>[2x]FPDGTLGMDAAVQEDHDNGTQLDSLTLASINTDFAFSLYKELVLKNPDTNIVFSPLSISAALALVSLGAKGNTLEEILEGLKFNLTETSEADIHQGFGHLLQRLNQPKDQVQISTGS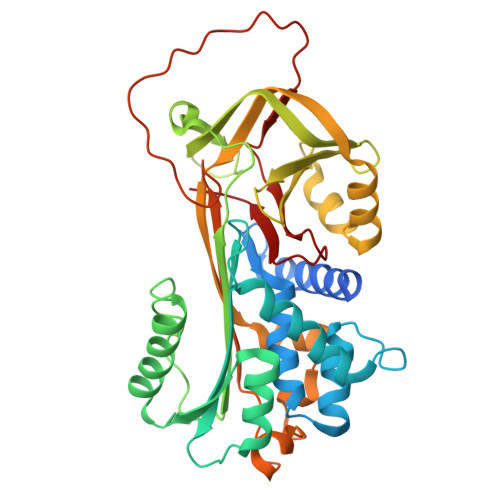ALFIEKRQQILTEFQEKAKTLYQAEAFTADFQQPRQAKKLINDYVRKQTQGMIKELVSDLDKRTLMVLVNYIYFKAKWKVPFDPLDTFKSEFYCGKRRPVIVPMMSMEDLTTPYFRDEELSCTVVELKYTGNASALFILPDQGRMQQVEASLQPETLRKWKNSLKPRMIDELHLPKFSISTDYSLEDVLSKLGIREVFSTQADLSAITGTKDLRVSQVVHKAVLDVAETGTEAAAATGVKFVPMSAKLYPLTVYFNRPFLIMIFDTETEIAPFIAKIANPK> GMTYQALMFDIDGTLTNSQPAYTTVMREVLATYGKPFSPAQAQKTFPMAAEQAMTELGIAASEFDHFQAQYEDVMASHYDQIELYPGITSLFEQLPSEL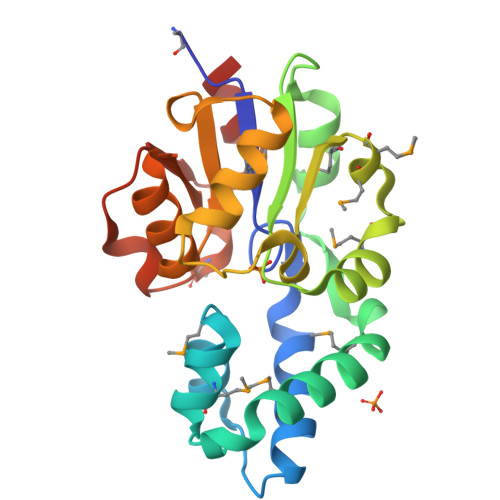RLGIVTSQRRNELESGMRSYPFMMRMAVTISADDTPKRKPDPLPLLTALEKVNVAPQNALFIGDSVSDEQTAQAANVDFGLAVWGMDPNADHQKVAHRFQKPLDILELFK> MQRNLTKLSAAAFYEFVDNNFLNNKRPPVPGGSWTVEVLRNKSLADLQHIWFLLLKERNMLKSMKEHYLRHQEELGAMPAPSRLKMIDESMRNIKRVVKERDEEATARAVEIFKERLKRGIYRYPPGPPPPPGAHDKTSVVKVELSCYVEEERLRELFGRYDVFEPHKGIVRVELKLPDEVLKQKEEAEQLWTQYMAECSDVKAYHQWSTAAPSAYDYTEVELAPGIFANDAISDKGGKHSGDTETHEGVIVAARVPVPPPKEKQPPPKNPLERLKAERRSYLARTTIQLGYFPNVTLPPPRYETVEAVPRPVHPDEIEGPWEAYITYDREDGLSYAQSLGITTIGVATVLGLTEHVREPQPYAVVDPVYCEALRRERAREETLMKWPHVPEWKYEY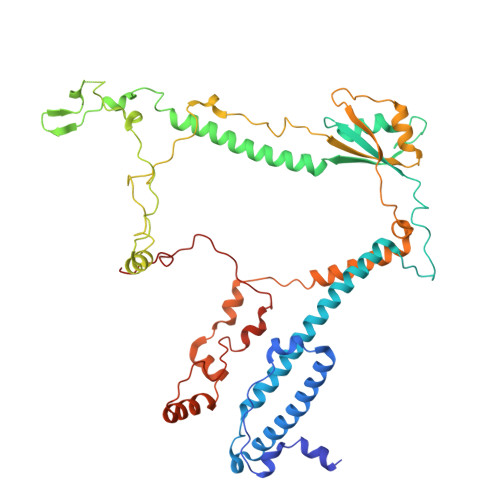STYTRKHLADIVQYNYTNVVDYVDREVLLTGKSVWECPIHIDHTCGGSKTVPPHAKKPVRYMDAGIANVGVTDI> MKVIFLKDVKGKGKKGEIKNVADGYANNFLFKQGLAIEATPANLKALEAQKQKEQRQAAEELANAKKLKEQLEKLTVTIPAKAGEGGRLFGSITSKQIAESL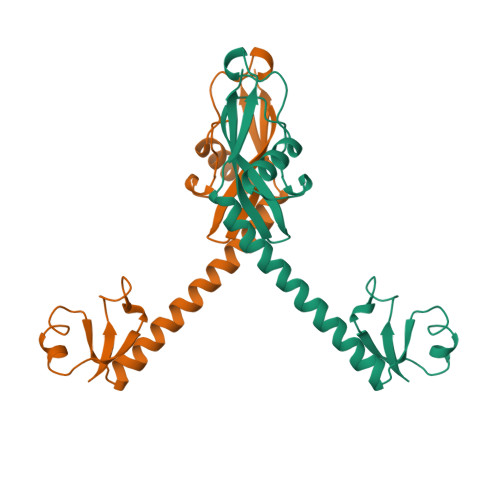QAQHGLKLDKRKIELADAIRALGYTNVPVKLHPEVTATLKVHVTEQK(2R)-2,3-dihydroxypropyl (9Z)-octadec-9-enoate | C21 H40 O4 | 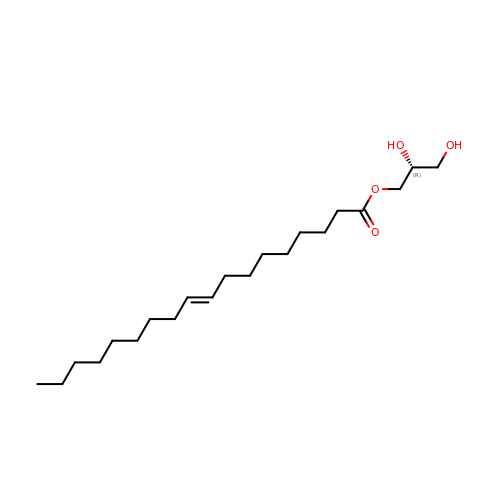RZRNAYUHWVFMIP-GDCKJWNLSA-N> HKCDITLQEIIKTLNSLTEQKTLCTELTVTDIFAASKNTTEKETFCRAATVLRQFYSHHEKDTRCLGATAQQFHRHKQLIRFL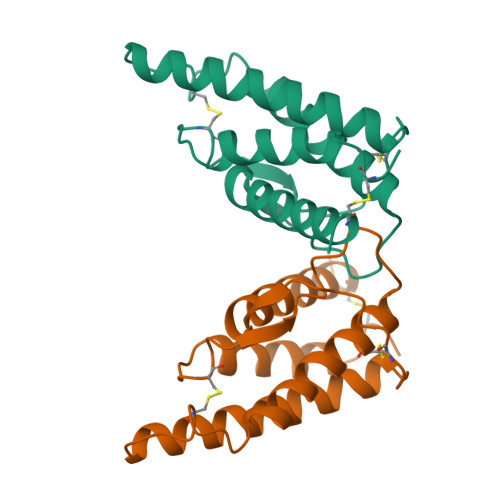KRLDQNLWGLAGLNSCPVKEANQSTLENFLERLKTIMREKYSKCSS>[2x]MSSLLNSLLPEYFKPKTNLNINSSRVQYGFNARIDMQYEDDSGTRKGSRPNAFMSNTVAFIGNYEGIIVDDIPILDGLRADIFDTHGDLDMGLVEDALSKSTMIRRNVPTYTAYASELLYKRNLTSLFYNMLRLYYIKKWGSIKYEKDAIFYDNGHACLLNRQLFPKSRDASLESSLSLPEAEIAMLDPGLEFPEEDVPAILWHGRVSSRATCILGQACSEFAPLAPFSIAHYSPQLTRKLFVNAPAGIEPSSGRYTHEDVKDAITILVSANQAYTDFEAAYLMLAQTLVSPVPRTAEASAWFINAGMVNMPTLSCANGYYPALTNVNPYHRLDTWKD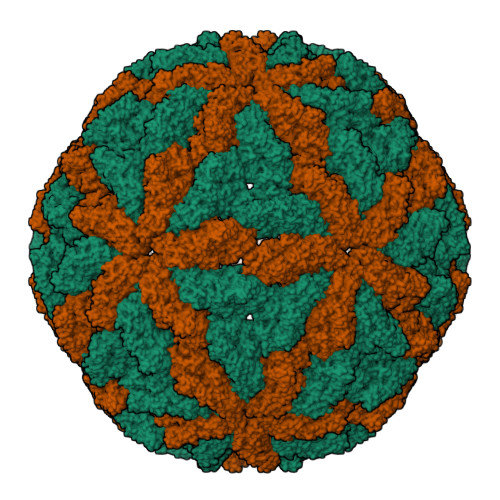TLNHWVAYPDMLFYHSVAMIESCYVELGNVARVSDSDAINKYTFTELSVQGRPVMNRGIIVDLTLVAMRTGREISLPYPVSCGLTRTDALLQGTEIHVPVVVKDIDMPQYYNAIDKDVIEGQETVIKVKQLPPAMYPIYTYGINTTEFYSDHFEDQVQVEMAPIDNGKAVFNDARKFSKFMSIMRMMGNDVTATDLVTGRKVSNWADNSSGRFLYTDVKYEGQTAFLVDMDTVKARDHCWVSIVDPNGTMNLSYKMTNFRAAMFSRNKPLYMTGGSVRTIATGNYRDAAERLRAMDETLRLKPFKITEKLDFRVAAYAIPSLSGSNMPSLHHQEQLQISEVDAEPINPIGEDELPPDIE>[2x]MAQERKVALVTGASRGIGAAIAQQLIQDGYFVVGTATSESGAQKLTDSFGEQGAGLALDVRNLDEIEAVVSHI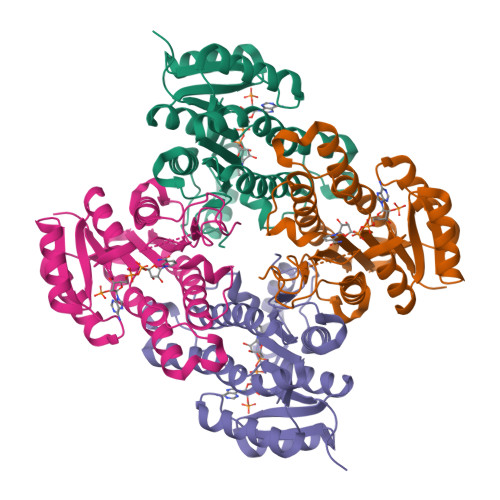EQNYGPVLVLVNNAGITKDNLLLRMSEDDWDDILNIHLKAVYRLSKRVLKGMTKARFGRIINISSVVAHFANPGQANYSAAKAGIEAFSRSLAKEMGSRQITVNSVAPGFIATEMTDALSEDIRKKMSDQVALNRLGEPQDIANAVSFLASDKAGYITGTVLHVNGGLYMA>MSSQFIFEDVPQRNAATFNPEVGYVAFIGKYGQQLNFGVARVFFLNQKKAKMVLHKTAQPSVDLTFGGVKFTVVNNHFPQYVSNPVPDNAITLHRMSGYLARWIADTCKASVLKLAEASAQIVMPLAEVKGCTWADGYTMYLGFAPGAEMFLDAFDFYPLVIEMHRVLKDNMDVNFMKKVLRQRYGTMTAEE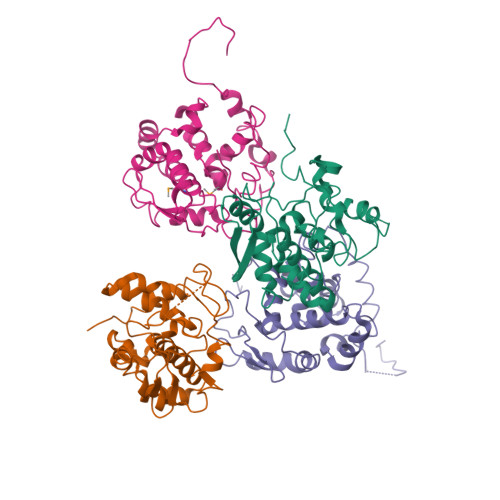WMTQKITEIKAAFNSVGQLAWAKSGFSPAARTFLQQFGINI[4x]> MKLNIAYPRNGTVKQFEISDEVLRRVQLQDYRLGNEVDGAIFGSEFKGYIFRLRGGSDKDGFPMVPGVLASS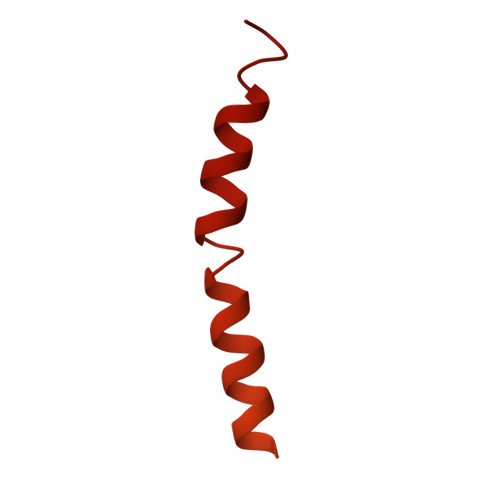RVSLLVKRGAIGFNTFRGYQGERRRKNVRGCVLASDIALVNVTISKVGDQPIEGVTDTTAPRRLGPKRASKIRKLFNLSRTEDVRKYVVRRRVVKSGKKDRLKAPKIQRLITPRVKARRAKKAKDAIAKVRASAAERREYLRLIASNRRALRQRDHSKKHTRKVHAQRAEVAAFQKK>MERLRQIASQATAASAAPARPAHPLDPLSTAEIKAATNTVKSYFAGKKISFNTVTLREPARKAYIQWKEQGGPLPPRLAYYVILEAGKPGVKEGLVDLASLSVIETRALETVQPILTVEDLCSTEEVIRNDPAVIEQCVLSGIPANEMHKVYCDPWTIGYDERWGTGKRLQQALVYYRSDEDDSQYSHPLDFCPIVDTEEKKVIFIDIPNRRRKVSKHKHANFYPKHMIEKVGAMRPEAPPINVTQPEGVSFKMTGNVMEWSNFKFHIGFNYREGIVLSDVSYNDHGNVRPIFHRISLSEMIVPYGSPEFPHQRKHALDIGEYGAGYMTNPLSLGCDCKGVIHYLDAHFSDRAGDPITVKNAVCIHEEDDGLLFKHSDFRDNFATSLVTRATKLVVSQIFTAANYEYCLYWVFMQDGAIRLDIRLTGILNTYILGDDEEAGPWGTRVYPNVNAHNHQHLFSLRIDPRIDGDGNSAAACDAKSSPYPLGSPENMYGNAFYSEKTTFKTVKDSLTNYESATGRSWDIFNPNKVNPYSGKPPSYKLVSTQCPPLLAKEGSLVAKRAPWASHSVNVVPYKDNRLYPSGDHVPQWSGDGVRGMREWIGDGSENIDNTDILFFHTFGITHFPAPEDFPLMPAEPITLMLRPRHFFTENPGLDIQPSYAMTTSEAKRAVHKETKDKTSRLAFEG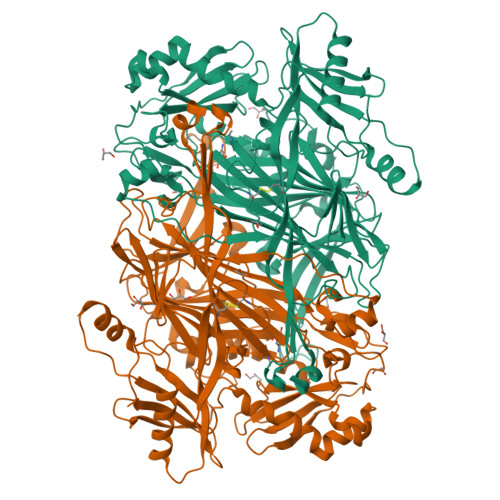SCCGK[6x]> GASGSMVEKNGAKKTSLRELPKISDRVSFIYVEHAKINRVDSAITVLDSRGTVRIPAAMIGVLLLGPGTDISHRAVELIGDTGTSMVWVGERGVRQYAHGRSLAHSTKFLEKQAKLVSNSRLRLAVARKMYQMRFPDEDVSAMTMQQLRGREGARVRRVYRLQSEKYQVSWTKREYNPDDFEGGDIV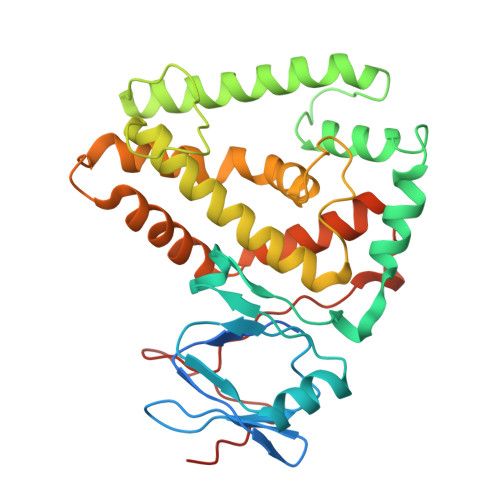NQALSAANVALYGLVHSIVIALGASPGLGFVHTGHDLSFIYDIADLYKAELTIPLAFEIAANFTEIDDIGKIARQKVRDSFVDGKLIVRIVQDIQYLFDLDDDEELLVDTLSLWDDKDMLVKHGVSYKEEL4-(1H-1,2,4-triazol-1-yl)phenol | C8 H7 N3 O | 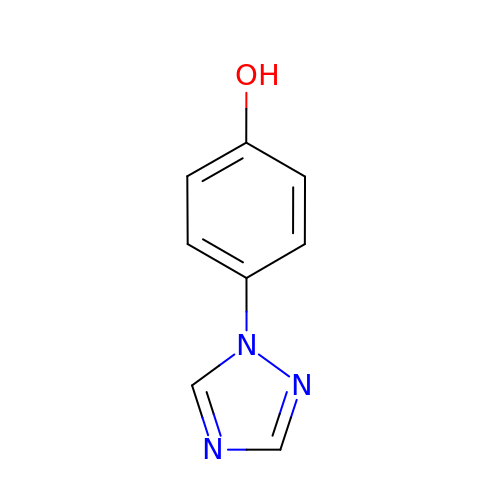ZOPIBCDDKMAEII-UHFFFAOYSA-N1-[5-chloranyl-4-(trifluoromethyl)-2,3-dihydroindol-1-yl]ethanone | C11 H9 Cl F3 N O | 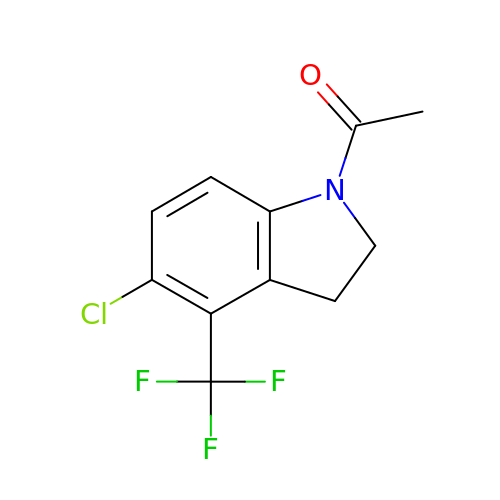OCTQANMBVHBRLQ-UHFFFAOYSA-N>YYIAIDIGGTQIKSAVIDKQLNMFDYQQISTPDNKSELITDKVYEIVTGYMKQYQLIQPVIGISSAGVVDEQKGEIVYAGPTIPNYKGTNFKRLLKSLSPYVKVKNDVNAALLGELKLHQYQAERIFCMTLGTGIGGAYKNNQGHIDNGELHKANEVGYLLYRPTENTTFEQRAATSALKKRMIAGGFTRSTHVPVLFEAAEEGDDIAKQILNEWAEDVAEGIAQIQVMYDPGLILIGGGISEQGDNLIKYIEPKVAH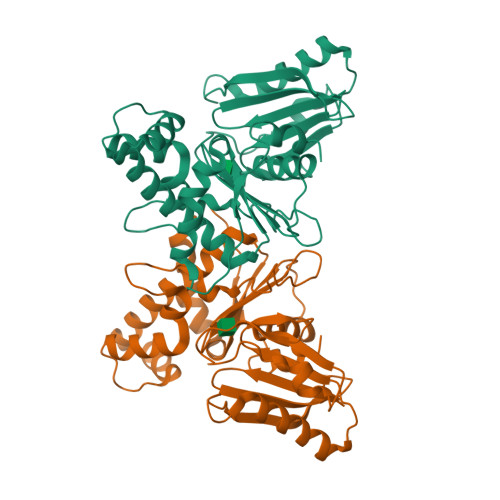YLPKDYVYAPIQTTKSKNDAALYGCLQ[4x]> MYIV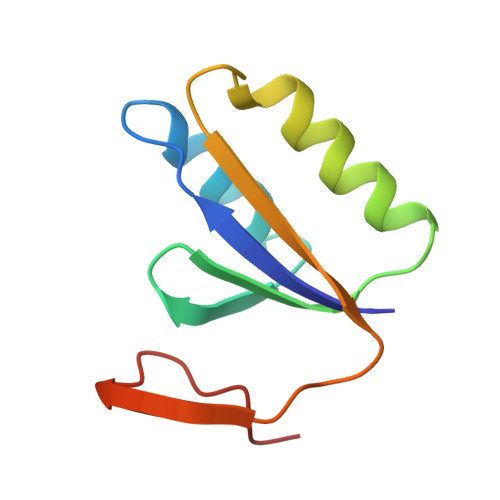VVYDVGVERVNKVKKFLRMHLNWVQNSVFEGEVTLAEFERIKEGLKKIIDENSDSVIIYKLRSMPPRETLGIEKNPIEEII>[2x]SKAKRLSSPRVRTHPMAPEKAEIFNSLHGWFEDNILPFLKPVEESWQPTDFLPDSTSDGFHQQVEELRRRTAELPDDYLVALV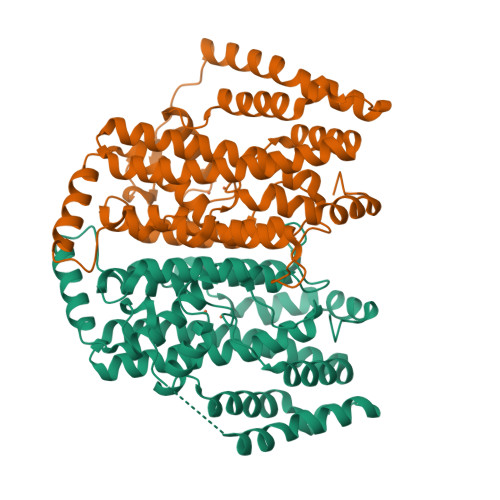GAMVTEEALPTYQTMLNTADVVHDESGASPLPWAVWTRAWTAEENRHGEIVNKYLYLSGRVDMKQIEKTIQYLIGSGMDPGTDNNPYLGFIYTSYQERATAISHGSLGRLARQKGELRLAQICGTISADEKRHEAAYTRIVEKLFEMDPEGTMLALEDMMKKKIVMPSHLMHDGKDPDLFQHFSAVSQRLGIYTAREYTDVLEHLIARWGVDKIMGLRDEGRRAQDYVCGLPSRFRRVEEKAQAWAEKVSHVPFSWVFGRTV> MIPPRFEYHAPKSVGEAVALLGQLGSDAKLLAGGHSLLPMMKLRFAQPEHLIDINRIPELRGIREEGSTVVIGAMTVENDLISSPIVQARLPLLAEAAKLIADPQVRNRGTIGGDIAHGDPGNDHPAL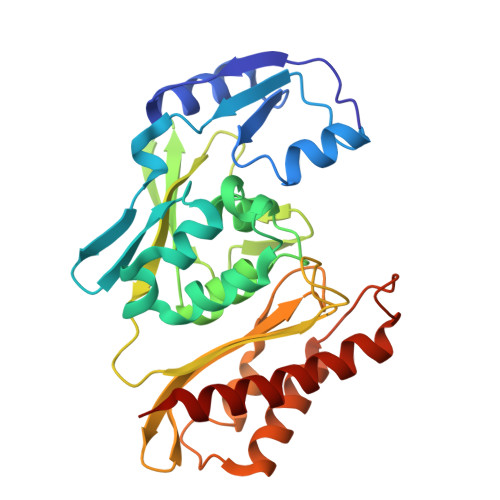SIAVEAHFVLEGPNGRRTVPADGFFLGTYMTLLEENEVMVEIRVPAFAQGTGWAYEKLKRKTGDWATAGCAVVMRKSGNTVSHIRIALTNVAPTALRAEAAEAALLGKAFTKEAVQAAADAAIAICEPAEDLRGDADYKTAMAGQMVKRALNAAWARCA>MATFPELLRPLKLGRYTLRNRIIMAPLTRCQATEDDHVPRTESMLKYYEDRASAGLIIAEATMVQPNYTGFLTEPGIYSDAQIEEWRKIVDAVHKKGGLIFLQLIHAGRAGIPEKILQQSKSDQDPLAGRLLAASAIPIKDHRIPAYFAASGEKETYGVPEELTDDEVRDGIIPLFVEGAKNAIFKAGFDGVEIHGANGYLLDAFFRESSNKRQSGPYAGTTIDTRCQLIYDVTKSVCDAVGSDRVGLRISPLNGVHGMIDSNPEALTKHLCKKIEPLSLAYLHYLRGDMVNQQIGDV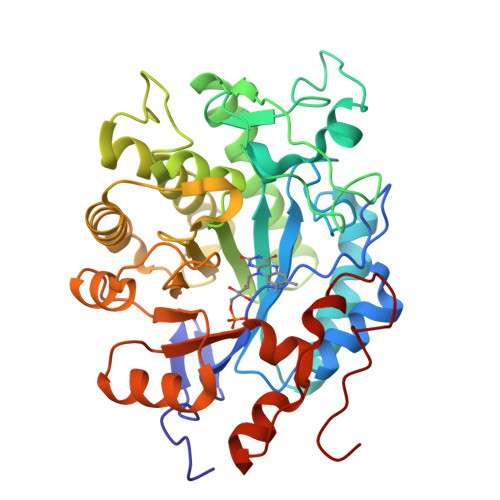VAWVRGSYSGVKISNLRYDFEEADQQIREGKVDAVAFGAKFIANPDLVERAQQNWPLNEPRPETYYTRTAVGYNDYPTYNK[2x]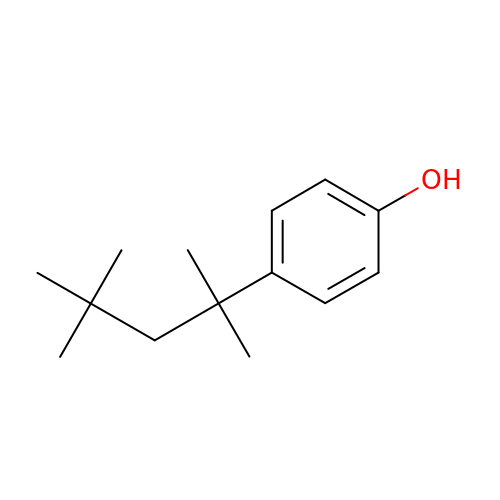4-(2,4,4-trimethylpentan-2-yl)phenol | C14 H22 O | ISAVYTVYFVQUDY-UHFFFAOYSA-N>[6x]EHNFNVVINAYDTTIPELNVEGVTVKNI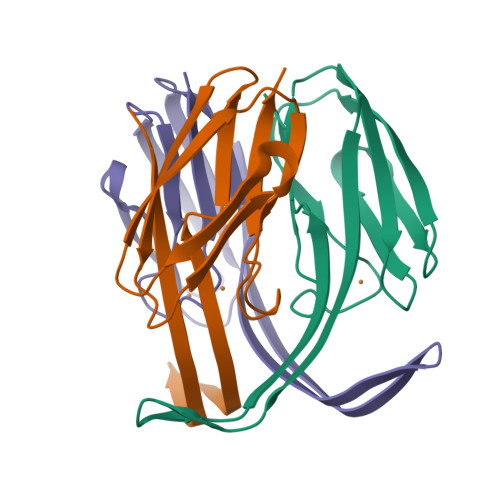RAFNVLNEPETLVVKKGDAVKVVVENKSPISEGFSIDAFGVQEVIKAGETKTISFTADKAGAFTIWCQLHPKNIHLPGTLNVVE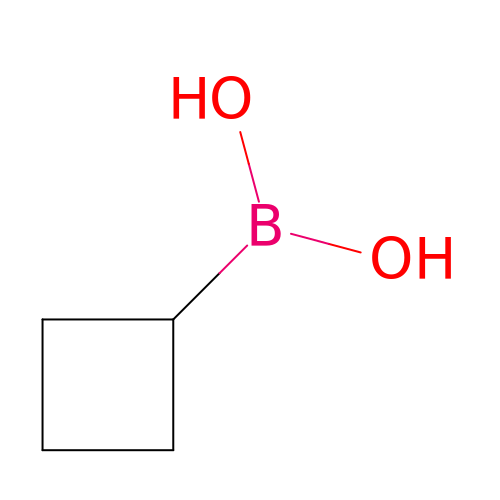cyclobutylboronic acid | C4 H9 B O2 | MIUALDDWOKMYDA-UHFFFAOYSA-N> GSHMASMTGGQQMGRGSEFRSMTAIEDILQITTDPSDTRGYSLLKSEEVPQGSTLGVDFIDTLLLYQLTENEKLDKPFEYLNDCFRRNQQQKRITKNKPNAESLHSTFQEIDRLVIGYGVVALQIENFCMNGAFINYITGIVSNVNSYTDFLSQIIQRAILEGTALDLLNAVFPTLLEYCNKHVSHFDLNESVIYNNVLTIFELFVTFKPIAEIFTKIDGFFADYSCKPQDFERKTILGPILSLSPIEAAVAIRNYGDNLLRSKQQTAMIHESLQAEHKVVIDRLFFIVDKLVRGSLNSRTDMISYFAHIANKNHLRRADHPPFKELSSNGFMSNITLLLVRFSQPFLDISYKKIDKIDANYFNNPSLFIDLSGETRLNSDFKEADAFYDKNRKTADSKPNFISDCFFLTLTYLHYGLGGTLSFEEKMGSEIKALKEEIEKVKKIAANHDVFARFITAQLSKMEKALKTTESLRFALQGFFAHRSLQLEVFDFICGASTFLIRVVDPEHEFPFKQIKLPLIPDQIGVENVDNADFLRAHAPVPFKYYPEFVVEGPVNYSLYISKYQTSPIFRNPRLGSFVEFTTMVLRCPELVSNPHLKGKLVQLLSVGAMPLTDNSPGFMMDIFEHDELVNKNLLYALLDFYVIVEKTGSSSQFYDKFNSRYSISIILEELYYKIPSYKNQLIWQSQNNADFFVRFVARMLNDLTFLLDEGLSNLAEVHNIQNELDNRARGAPPTREEEDKELQTRLASASRQAKSSCGLADKSMKLFEIYSKDIPAAFVTPEIVYRLASMLNYNLESLVGPKCGELKVKDPQSYSFNPKDLLKALTTVYINLSEQSEFISAVAKDERSFNRNLFVRAVDILGRKTGLASPEFIEKLLNFANKAEEQRKADEEEDLEYGDVPDEFLDPLMYTIMKDPVI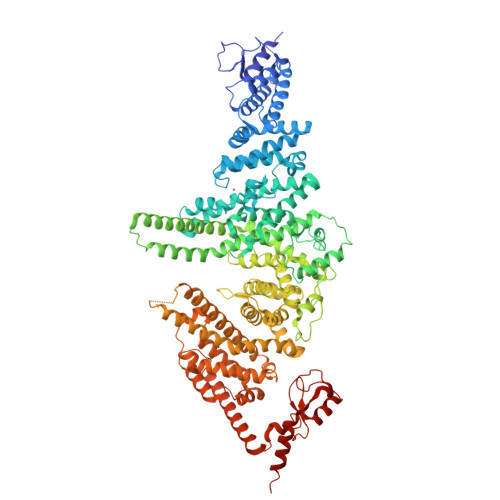LPASKMNIDRSTIKAHLLSDSTDPFNRMPLKLEDVTPNEELRQKILCFKKQKKEEAKHKASE> SFRTDKKPDPANWEYKSLYRGDIARYKRKGDSCLGINPKKQCISWEGTSTEKKHSRKQVERYFTKKSVGLMNIDGVAISSKTEPPSSEPISFIPVKDLEDAAPVT;> GAMDPEFTDEPIFGKKPRIEESITEDLSLADLMPRVKVQSVETVEGCTHEVALPAEEDYLPLKPRVGKAAKEYPFILDAFQREA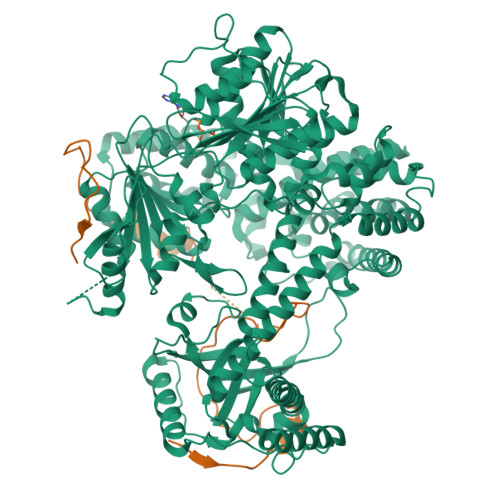IQCVDNNQSVLVSAHTSAGKTVCAEYAIALALREKQRVIFTSPIKALSNQKYREMYEEFQDVGLMTGDVTINPTASCLVMTTEILRSMLYRGSEVMREVAWVIFDEIHYMRDSERGVVWEETIILLPDNVHYVFLSATIPNARQFAEWICHLHKQPCHVIYTDYRPTPLQHYIFPAGGDGLHLVVDENGDFREDNFNTAMQVLRDAGDLAKGDQKGRKGGTKGPSNVFKIVKMIMERNFQPVIIFSFSKKDCEAYALQMTKLDFNTDEEKKMVEEVFSNAIDCLSDEDKKLPQVEHVLPLLKRGIGIHHGGLLPILKETIEILFSEGLIKALFATETFAMGINMPARTVLFTNARKFDGKDFRWISSGEYIQMSGRAGRRGMDDRGIVILMVDEKMSPTIGKQLLKGSADPLNSAFHLTYNMVLNLLRVEEINPEYMLEKSFYQFQHYRAIPGVVEKVKNSEEQYNKIVIPNEESVVIYYKIRQQLAKLGKEIEEYIHKPKYCLPFLQPGRLVKVKNEGDDFGWGVVVNFSKKSNVKPNSGELDPLYVVEVLLRCSKESLKNSATEAAKPAKPDEKGEMQVVPVLVHLLSAISSVRLYIPKDLRPVDNRQSVLKSIQEVQKRFPDGIPLLDPIDDMGIQDQGLKKVIQKVEAFEHRMYSHPLHNDPNLETVYTLCEKKAQIAIDIKSAKRELKKARTVLQMDELKCRKRVLRRLGFATSSDVIEMKGRVACEISSADELLLTEMMFNGLFNDLSAEQATALLSCFVFQENSSEMPKLTEQLAGPLRQMQECAKRIAKVSAEAKLEIDEETYLSSFKPHLMDVVYTWATGATFAHICKMTDVFEGSIIRCMRRLEELLRQMCQAAKAIGNTELENKFAEGITKIKRDIVFAASLYL5-(1H-benzimidazol-2-yl)-2,4-dihydro-3H-1,2,4-triazol-3-one | 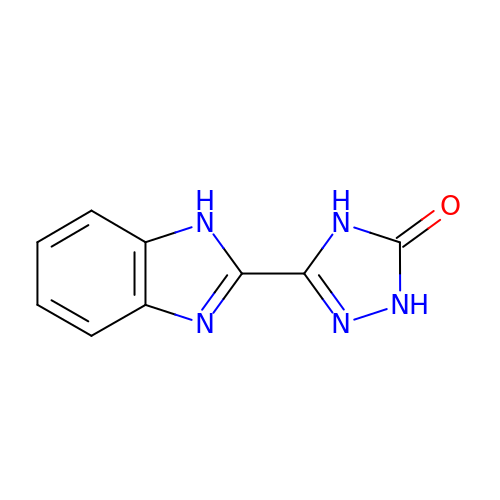C9 H7 N5 O | RSNCHZFKYVCLEY-UHFFFAOYSA-N>GAVPELGSREIEILGESVVLVTAYDENRKVVSQGSGFAVGTGLFATNYHLVKDGVVVKITAGDGKVYDVDGIVKYDKAKDLALLKTTVETGVNPLKLGTKKSLTKGSRIVAIGKANGAKNTVTKGSIKSLKVDGLTDAIELSASISKESTGGPVFDMKGNVVGITAYGISKQNVNAVIPADYVADWVKELSKHSFGNIRIVRKTLVFDSDFEFNFVVYKIIRALENEDAATYFGCMTDELYKDETRKNLEVLFTTYDLAYNIESINVVSKSEEQAKVSYVYTINKEAGPNFKNYRIIGECSLIKVDGTWKINDSE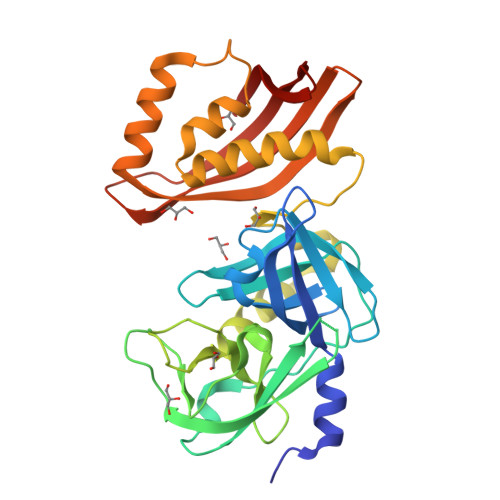EK[2x]>[2x]MPIMLEDYQKNFLEL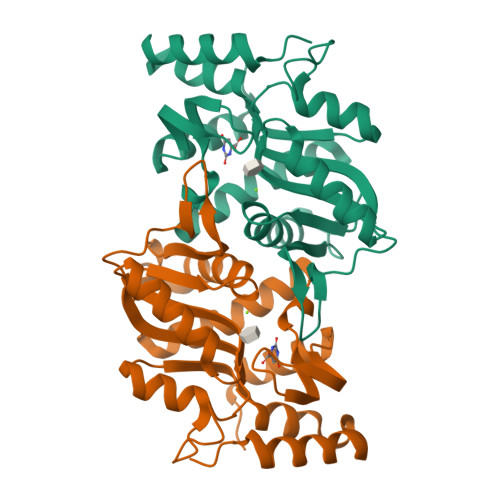AIECQALRFGSFKLKSGRESPYFFNLGLFNTGKLLSNLATAYAIAIIQSDLKFDVIFGPAYKGIPLAAIVCVKLAEIGGSKFQNIQYAFNRKEAKDHGEGGIIVGSALENKRILIIDDVMTAGTAINEAFEIISNAKGQVVGSIIALDRQEVVSTDDKEGLSATQTVSKKYGIPVLSIVSLIHIITYLEGRITAEEKSKIEQYLQTYGASA>[12x]GAMDAEGLALLLPPVTLAALVDSWLREDCPGLNYAALVSGAGPSQAALWAKSPGVLAGQPFFDAIFTQLNCQVSWFLPEGSKLVPVARVAEVRGPAHCLLLGERVALNTLARCSGIASAAAAAVEAARGAGWTGHVAGTRKTTPGFRLVEKYGLLVGGAASHRYDLGGLVMVKDNHVVAAGGVEKAVRAARQAADFALKVEVECSSLQEAVQAAEAGADLV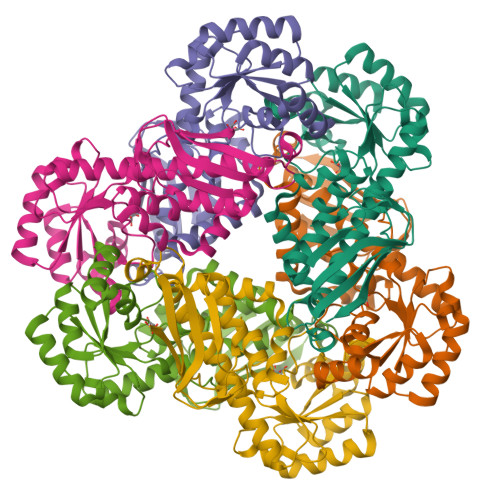LLDNFKPEELHPTATVLKAQFPSVAVEASGGITLDNLPQFCGPHIDVISMGMLTQAAPALDFSLKLFAKEVAPVPKIH>[3x]QQIGTIPEVHPKLPTWKCTTEGGCVQQNTSVVLEYLSHPIHEVGNSDVSCVVSGGLNQSLCPNEEECSKNCVVEGANYTSSGVHTDGDALTLNQYVTNGDQVVTASPRVYLLASDDEDGNYSMLQLLGQELSFDV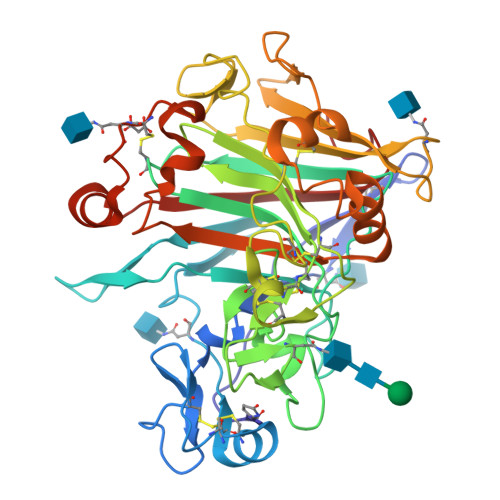DVSKLVCGMNGALYLSEMDASGGRNSLNPAGAQYGSGYCDAQCGVQPFINGTVNTGSLGACCNEMDIWEANALATALTPHPCSVTSIYACSGAECGSNGVCDKPGCGYNPYALGDHNYYGPGKTVDTSRPFTVVTQFLTNDNTTTGTLTEIRRLYVQDGNVIGPSPSDSVSSITDSFCSTVDSYFEPLGGLKEMGEALGRGMVLVFSIWNDPGQFMNWLDSGNAGPCNSTEGNPATIEAQHPDTAVTFSNIRWGDIGSTFQS>[2x]MGSSHHHHHHSSLVPRGSHMASQSMITPTTQIAGAGVLGNDRKPDESCARAAAAADPGPPTRPAHNAAGVSPEMVQVPAEAQRIVVLSGDQLDALCALGLQSRIVAAALPNSSSSQPSYLGTTVHDLPGVGTRSAPDLRAIAAAHPDLILGSQGLTPQLYPQLAAIAPTVFTAAPGADWENNLRGVGAATARIAAVDALITGFAEHATQVGTKHDATHFQASIVQLTANTMRVYGANNFPASVLSAVGVDRPPSQRFTDKAYIEIGTTAADLAKSPDFSAADADIVYLSCASEAAAERAAVILDSDPWRKLSANRDNRVFVVNDQVWQTGEGMVAARGIVDDLRWVDAPIN

Mtb FecB and FecB2 are predicted periplasmic binding proteins implicated in host iron acquisition; however, their precise roles are not well understood. In vitro ligand binding experiments for FecB and FecB2 were performed with heme and bacterial siderophores from Mtb and other species, revealing that both FecB and FecB2 bind heme, while only FecB binds the Mtb sideophore ferric-carboxymycobactin (Fe-cMB). Mtb FecB and FecB2 are both members of the type III PBP family. Each protein structure is composed of N- and C-terminal lobes consisting of mixed α/β structures with a central β-sheet surrounded by α-helices, with the two lobes linked by a rigid “backbone” helix (α6), forming the characteristic fold of the type III PBP family.

The structure of FecB was solved to 2.0 Å in space group C2, and the asymmetric unit contains two FecB molecules (chain A, 42–356 and chain B, residues 45–357, where numbering is for the unprocessed FecB form). Notably, FecB has an extra N-terminal sequence that associates with the C-terminal lobe but has an unstructured connection between the N- and C-terminal lobes (dashed black line). The substrate binding pocket of FecB is quite different from that of FecB2 in contributing residues, shape, and electrostatic charges. The FecB binding pocket has three tyrosine, four asparagine, three glutamine and two arginine residues along with a glutamate and aspartate residue, Figs 2A and 3. The binding cleft of FecB2 contains three arginine and two glutamine residues along with one glutamate, aspartate and tyrosine residue to provide polar contacts with a bound ligand; and three tryptophan and three phenylalanine residues. The resulting FecB pocket is narrower and deeper than the FecB2 ligand-binding pocket, with one side pinched together creating an almost triangular chasm, Fig 2. In contrast, the back of the FecB pocket is negatively charged. Indeed, this charged environment trapped a polyethylene glycol molecule from the crystallographic condition. Mtb FecB has highest structural similarity to ferric-siderophore binding proteins such as Bacillus cereus YfiY (2.5 Å rmsd), Staphylococcus aureus SirA (3.1 Å rmsd) and HtsA (3.6 Å rmsd). Out of the ten variants tested (R141S, L163R, Q233S, R240S, Y242S, Y270S, E272S, D322S, Q336S, and E339S), there was only one variant, E339S, that had a considerably reduced affinity to Fe-cMB. Ultimately, the affinity of the E339S variant was so diminished that it was unmeasurable due to the solubility limits of Fe-cMB. This acidic residue, Glu339, is situated at the back of the FecB ligand binding pocket.> GSHMLKDSLRPKLSEEQQHIIAILLDAHHKTYDPTYADFRDFRPPVRMDGSTGSVTLDLSPLSMLPHLADLVSYSIQKVIGFAKMIPGFRDLTSDDQIVLLKSSAIEVIMLRSNQSFTMDDMSWDCGSQDYKYDVTDVSKAGHTLELIEPLIKFQVGLKKLNLHEEEHVLLMAICIVSPDRPGVQDAKLVEAIQDRLSNTLQTYIRCRHPPPGSHQLYAKMIQKLADLRSLNEEHSKQYRSLSFQPEN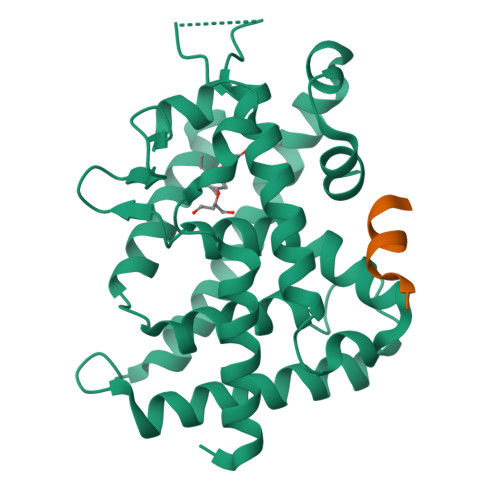SMKLTPLVLEVFGNEIS;> KNHPMLMNLLKDN>MATTSHQPQDRYKAVWLIFFMLGLGTLLPWNFFMTATQYFTNRLDMSQNVSLVTAELSKDAQASAAPAAPLPERNSLSAIFNNVMTLCAMLPLLLFTYLNSFLHQRIPQSVRILGSLVAILLVFLITAILVKVQLDALPFFVITMIKIVL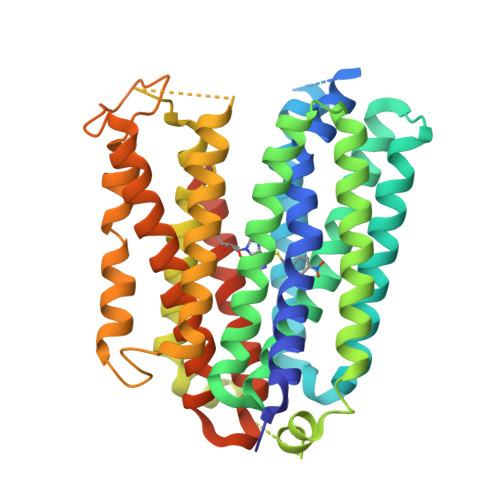INSFGAILQGSLFGLAGLFPASYTAAIMSGQGLAGFFASVAMICAIASGSELSESAFGYFITACAVIILTIICYLGLPRLEFYRYYQQLKLEGPTNESHSIKAILKKISVLAFSVCFIFTITIGMFPAVTVEVKSSIAGSSTWERYFIPVSCFLTFNIFDWLGRSLTAVFMWPGKDSRWLPSLVLARLVFVPLLLLCNIKPRRYLTVVFEHDAWFIFFMAAFAFSNGYLASLCMCFGPKKVKPAEAETAGAIMAFFLCLGLALGAVFSFLFRAIVGTELLQVDTNSLEVLFQ[2x]> MKTSDANETEDHLESLICKVGEKSACSLESNLEGLAGVLEADLPNYKSKILRLLCTVARLLPEKLTIYTTLVGLLNARNYNFGGEFVEAMIRQLKESLKANNYNEAVYLVRFLSDLVNCHVIAAPSMVAMFENFVSVTQEEDVPQVRRDWYVYAFLSSLPWVGKELYEKKDAEMDRIFANTESYLKRRQKTHVPMLQVWTADKPHPQEEYLDCLWAQIQKLKKDRWQERHI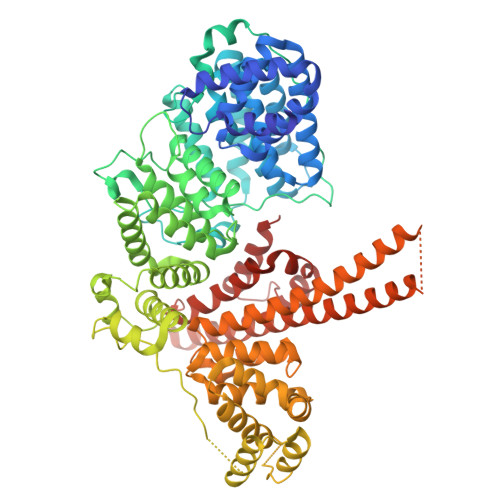LRPYLAFDSILCEALQHNLPPFTPPPHTEDSVYPMPRVIFRMFDYTDDPEGPVMPGSHSVERFVIEENLHCIIKSHWKERKTCAAQLVSYPGKNKIPLNYHIVEVIFAELFQLPAPPHIDVMYTTLLIELCKLQPGSLPQVLAQATEMLYMRLDTMNTTCVDRFINWFSHHLSNFQFRWSWEDWSDCLSQDPESPKPKFVREVLEKCMRLSYHQRILDIVPPTFSALCPVNPTCIYKYGDESSNSLPGHSVALCLAVAFKSKATNDEIFSILKDVPNPNQDDDDDEGFSFNPLKIEVFVQTLLHLAAKSFSHSFSALAKFHEVFKTLAESDEGKLHVLRVMFEVWRNHPQMIAVLVDKMIRTQIVDCAAVANWIFSSELSRDFTRLFVWEILHSTIRKMNKHVLKIQKELEEAKEKLARQHKRRSDDDDRSSDRKDGVLEEQIERLQEKVESAQSEQKNLFLVIFQRFIMILTEHLVRCETDGTSVLTPWYKNCIERLQQIFLQHHQIIQQYMVTLENLLFTAELDPHILAVFQQFCALQA> TVEKSVVFKAEGEHFTDQKGNTIVGSGSGGTTKYFRIPAMCTTSKGTIVVFADARHNTASDQSFIDTAAARSTDGGKTWNKKIAIYNDRVNSKLSRVMDPTCIVANIQGRETILVMVG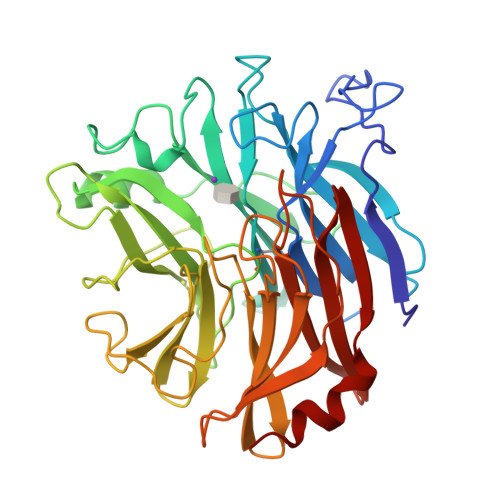KWNNNDKTWGAYRDKAPDTDWDLVLYKSTDDGVTFSKVETNIHDIVTKNGTISAMLGGVGSGLQLNDGKLVFPVQMVRTKNITTVLNTSFIYSTDGITWSLPSGYCEGFGSENNIIEFNASLVNNIRNSGLRRSFETKDFGKTWTEFPPMDKKVDNRNHGVQGSTITIPSGNKLVAAHSSAQNKNNDYTRSDISLYAHNLYSGEVKLIDDFYPKVGNASGAGYSCLSYRKNVDKETLYVVYEANGSIEFQDLSRHLPVIKSYN> MGANDYVPSPITINTSTLPVVVIGPADAHTYPRVIGELTGTSNQYIFNGGSLIALMRGKFTPTLPKIGKITYNFRQGNNTQSSDFDIFDTGVPGLGIIIGMAGYWPATPLVPINSSSIYIDPVAANTNPNAYNGATGSFGARLYVAFVATGRLPNGYVTIPTKQLGHILLESNRASLNNKRLTAPVMLNGGRIQVQSLEHHHHHH

Ucl fimbriae are attachment organelles that facilitate ExPEC adherence. Ucl fimbriae are phylogenetically related to Uca fimbriae from Proteus mirabilis and F17/G fimbriae from enterotoxigenic E. coli (ETEC). Tip adhesins are two-domain proteins; they possess a C-terminal pilin domain that connects the adhesin to the main fimbrial shaft, and an N-terminal lectin domain that mediates attachment to specific ligands, therefore dictating host range and tissue tropism.

Given the close phylogenetic relationship between the Ucl fimbriae and the Uca fimbriae from P. mirabilis, in parallel we also determined the crystal structure of UcaDLD (84% amino acid identity to UclDLD) at 1.6 Å resolution. The model was then used as a template for solving the structure of UcaDLD by molecular replacement. The final UclDLD and UcaDLD models contain residues 21–215 and 21–217, respectively. Electron density was not observed for residues 43–48 (UclDLD) and 44–47 (UcaDLD), suggesting that these regions have a disordered or flexible conformation in the crystals. As expected from the high sequence identity, the two structures are similar, with r.m.s.d. of 0.6 Å for 189 equivalent Cα atoms. A search for structures similar to UclD and UcaD in the PDB using the DALI server revealed significant similarity to F17G like adhesins (Z-score of 14.3–15.8 when using UcaDLD as the search model), although the sequence identity is only 14–16%. UclDLD and UcaDLD have a completely conserved pocket in the same region of the structure as the N-acetylglucosamine (GlcNAc)-binding site in F17G. The pocket also contains a tryptophan residue, which is known to mediate CH-π stacking interactions in the interaction site of other carbohydrate-binding proteins. By contrast, UcaDLD bound specifically to ten glycans from the glycan array, all but one of which, surprisingly, were different to the glycans bound by UclDLD. Binding for UcaD showed little direct overlap with UclD, with the highest affinity binding identified for UcaD being to neutral glycans containing GalNAc on the glycan core and sulfated Galβ1-4GlcNAc structures.>GPMVSEQSEIVTSKYQKIAVAVAQRIANGDYEVGEKLKSRTTIASTFNVSPETARKGLNILADLQILTLKHGSGAIILSKEKAIEFLNQYETSHSVAILKGKIRDNIKAQQQEMEELATLVDDFLLQTRAVSKQYPLAPYEIIVSEDSEHLGKSIGELNVWHQTGATIVAIEHEGKFIVSPGPFSVIEQGDHIFFVGDEDVYARMKTYFNL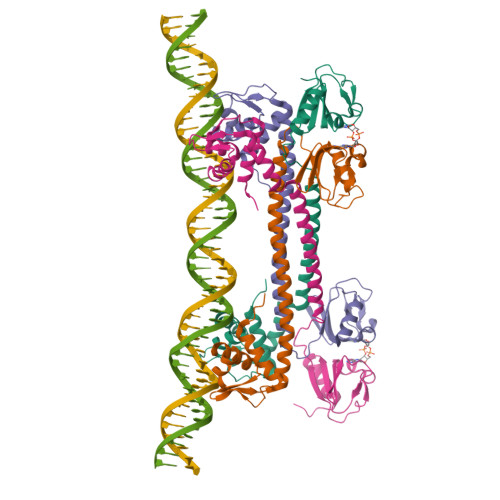RMGL[4x]>GAMAIEFNI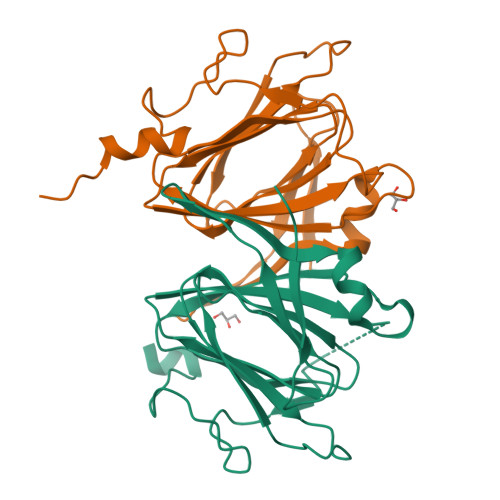QESKILKGVYIITPNKFRDLRGEIWTAFTSKAVDKLLPNGLKFIHDKFIHSKHNVIRGIHGDVKTYKLATCVYGEIHQVVVDCRKDSPTYLKYEKFIINQDNQQIILVPAGFGNAHYVTSESAVYYYKCAYKGDYVDAPDQFTYAWNDERIGIDWPTNSPILSERDILATKNKG[2x]> GAMISQPQEPELMNANPSPPPSPSQQINLGPSSNPHAKPSDFHFLKVIGKGSFGKVLLARHKAEEVFYAVKVLQKKAILKKKEEKHIMSERNVLLKNVKHPFLVGLHFSFQTADKLYFVLDYINGGELFYHLQREA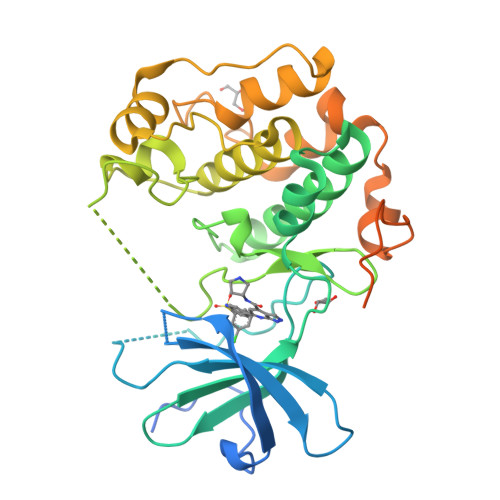CFLEPRARFYAAEIASALGYLHSLNIVYRDLKPENILLDSQGHIVLTDFGLCKENIEHNSTTSTFCGTPEYLAPEVLHKQPYDRTVDWWCLGAVLYEMLYGLPPFYSRNTAEMYDNILNKPLQLKPNITNSARHLLEGLLQKDRTKRLGAKDDFMEIKSHVFFSLINWDDLINKKITPPFNPNVSGPNDLRHFDPEFTEEPVPNSIGKSPDSVLVTASVKEAAEAFLGFDYAPPTDSFL The EphA4 tyrosine kinase cell surface receptor regulates an array of physiological processes and is the only currently known class A Eph receptor that binds both A and B class ephrins with high affinity. Eph receptors are type 1 membrane proteins with an N-terminal extracellular region consisting of a ligand binding domain (LBD), a cysteine rich region, and two fibronectin type III domains. We have solved the crystal structure of the EphA4 ligand binding domain alone and in complex with (1) ephrinB2 and (2) ephrinA2. Structural analyses, drawing on previously reported Eph receptor structures, show that EphA4 in isolation and in complex with ephrinA2 resembles other class A Eph receptors but on binding ephrinB2 assumes structural hallmarks of the class B Eph receptors. This interactive plasticity reveals EphA4 as a structural chameleon, able to adopt both A and B class Eph receptor conformations, and thus provides a molecular basis for EphA-type cross-class reactivity.

The flexibility inherent in these regions is consistent with their relatively high average crystallographic main chain B factor values in comparison with the rest of the protein (for our high resolution structures an average of 62 Å2 in BC, DE, GH, and JK loops versus 31 Å2 over the entire molecule). Given that the DE and JK loops map to regions in EphA2 and EphB2 crystal structures (Himanen et al., 2001), which move upon binding to their respective ephrin ligands, their flexibility may be of direct functional relevance. While ephrins generally exhibit a low degree of structural variance between different bound forms, structural analysis of EphA4 reveals distinct structural differences between unbound EphA4 and its ephrinA2 (1.7 Å rmsd over 166 equivalent Cα atoms)- and ephrinB2 (2.3 Å rmsd over 168 equivalent Cα atoms)-bound states. Most notable are the structural changes that occur to the DEEphA4 and JKEphA4 loops; regions which we identify above as having a high degree of flexibility in unbound EphA4. The structural differences between the two available apo LBD structures of EphA4 and the divergence in conformational changes that occur upon ephrinB2 and ephrinA2 binding are consistent with the EphA4 receptor maintaining a high degree of structural plasticity in its DEEphA4 and JKEphA4 ephrin binding loops. Other EphA receptor structures, including the apo and ephrinA2-bound EphA4 structures, on the other hand, are more distantly related to B class Eph receptors. However, inspection of the EphA2 unbound structures deposited by the Structural Genomics Consortium (Toronto) indicates that for these crystal structures the primary EphA2 ligand binding loops (JK and DE loops) are partially disordered or are in conformational states quite different to their bound forms.

>ETGEVTLLDSRSVQGELGWIASPLEGGWEEVSIMDEKNTPIRTYQVCNVMEPSQNNWLRTDWITREGAQRVYIEIKFTLRDCNSLPGVMGTCKETFNLYYYESDNDKERFIRENQFVKIDTIAADESFTQVDIGDRIMKLNTEIRDVGPLSKKGFYLAFQDVGACIALVSVRVFYKRTKHHHHHH[2x]> MRAMERTYTLVIGRPVVIGEKPVNIEKFANTSKGDAYEIKDLHIEFNVKKDNSKEPNKGYVTVYNLSDEVVNYLSVNQ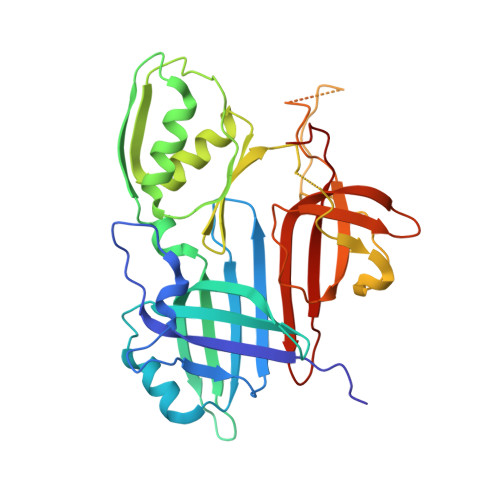RESLAVMLHAGYNGDEKLIFSGTVEYVEDDFPEETRTTKFILGDGTLNLTTATTARSYRKGTPVNSVLNDLIADLKLPKGRVIDFGNQTLQTSMAFTGNASQNLANLAKNTGSTFSVQDGAVYWTKEGSRFNNVMFEISEEGGMVGTPTPKQPSSSKKLIKAKAKAKSDEAEGKKPKAPSKKKKEHDIKEDVGMTVSTLLNGAILPESTVYLNTRYHKGFYKVAELTHRGGYETGDWITELGLVETRGELIK>CGCG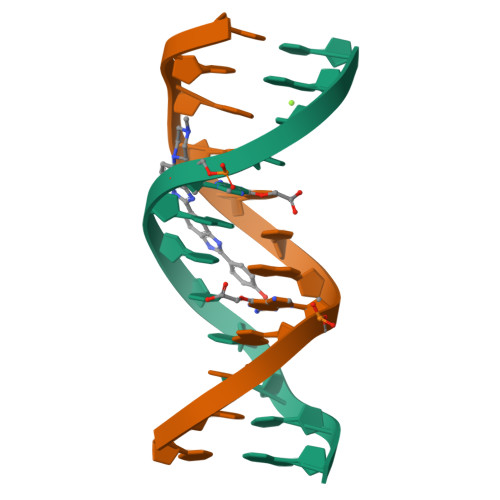XATTCGCG[2x]4-NITROPHENYL METHANETHIOL | C7 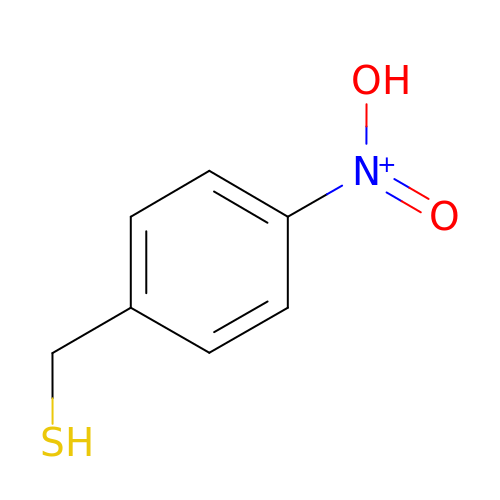H8 N O2 S | OTHKGVFNUSHUQO-UHFFFAOYSA-O>[4x]MLTSSSHHGRSYDVFLSFRGEDTRKTFVGHLFNALIEKGIHTFMDDKELKRGKSISSELMKAIGESRFAVVVFSKNYASSTWCLEELVKILEIHEKFELIVVPVFYDVDPSTVRKQNGEYAVCFTKFEANLVDDRDKVLRWREALTKVANISGHDLRNTYNGDESKCIQQILKDIFDKFCFSISITNRDLVGIESQIKKLSSLLRMDLKGVRLVGIWGMGGVGKTTAARALFNRYYQNFESACFLEDVKEYLQHHTLLYLQKTLLSKLLKVEFVDCTDTEEMCVILKRRLCSKKVLVVLDDVNHNDQLDKLVGAEDWFGSGSRIVITTRDMKLLKNHDVHETYEIKVLEKDEAIELFNLHAFKRSSPEKEFKELLNLVVDYTGGLPLALKVLGSLLYKEDLDVWISTIDRLKDNPEGEIMATLKISFDGLRDYEKSIFLDIACFFRGYNQRDMTALFHASGFHPVLGVKTLVEKSLIFI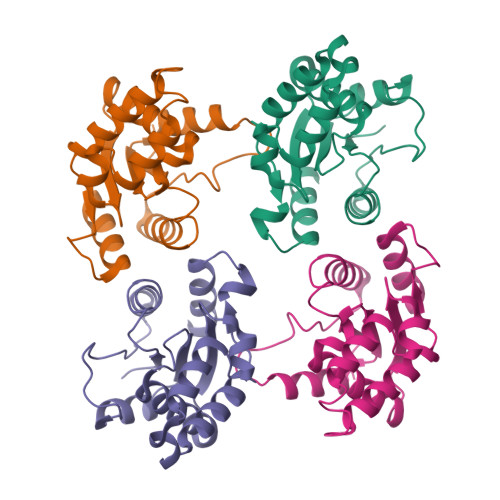LEDKIQMHDLMQEMGRQIAVQESPMRRIYRPEDVKDACIGDMRKEAIEGLLLTEPEQFEEGELEYMYSAEALKKTRRLRILVKEYYNRGFDEPVAYLPNSLLWLEWRNYSSNSFPSNFEPSKLVYLTMKGSSIIELWNGAKRLAFLTTLDLSYCHKLIQTPDFRMITNLERLILSSCDALVEVHPSVGFLKNLILLNMDHCISLERLPAIIQSECLEVLDLNYCFNLKMFPEVERNMTHLKKLDLTSTGIRELPASIEHLSSLENLQMHSCNQLVSLPSSIWRFRNLKISECEKLGSLPEIHGNSNCTRELILKLVSIKELPTSIGNLTSLNFLEICNCKTISSLSSSIWGLTSLTTLKLLDCRKLKNLPGIPNAINHLSGHGLQLLLTLEQPTIYERLDLLRIIDMSWCSCISSLPHNIWMLKFLRILCISYCSRLEYLPENLGHLEHLEELLADGTGILRLPSSVARLNKLEVLSFRKKFAIGPKVQYSSSMLNLPDDVFGSLGSLGSVVKLNLSGNGFCNLPETMNQLFCLEYLDITFCQRLEALPELPPSIKELYVDEHLALRIMEDLVIKCKELNLIAVTKIEYQNFYRWLDSIWSDVSELLENSQKQQLDDMLQLIPFSYLSTAKREEVLKIVIHGTRIPEWFRWQDRSATTMSVNLPEYWYTENFLGFAICCSCCFYHSARSYDVEFEGSMHHYNYDSSYWKEYEEPSYDFYERDSIEITAKLTPRHKGMRTEELKKVCSFSMNVLRRATAVPNMCFAFFPFNSLCHISNLQANNPNDYGIFETCLSPGDIRHRGKQWGFNLVYKDETGGSVTHEMLINRDYKDHDGDYKDHDIDYKDDDDK> MDEPLSILVRNNKGRSSTYEVRL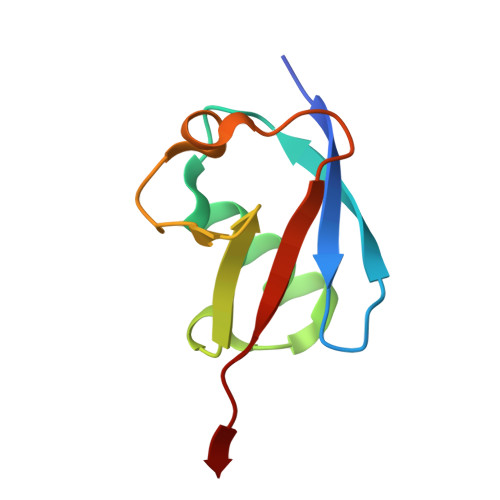TQTVAHLKQQVSGLEGVQDDLFWLTFEGKPLEDQLPLGEYGLKPLSTVFMNLRLRG> KIPEHLIGKGAEADIKRDSYLDFDVIIKERVKKGYRDERLDENIRKSRTAREARYLALVKDFGIPAPYIFDVDLDNKRIMMSYINGKLAKDVIEDNL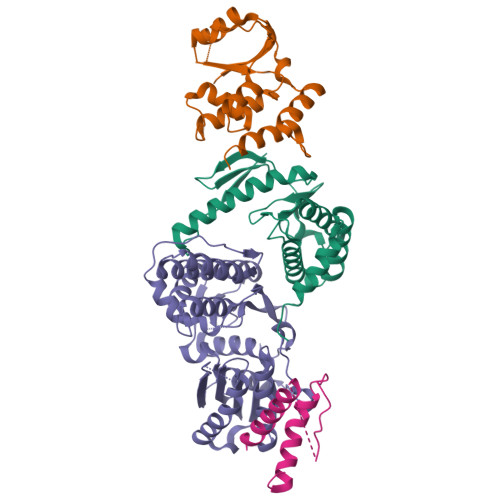DIAYKIGEIVGKLHKNDVIHNDLTTSNFIFDKDLYIIDFGLGKISNLDRDKAVDLIVFKKAVLSTHHEKFDEIWERFLEGYKSVYDRWEIILELMKDVERRARYVE;> PMIIRGIRGARINNEIFNLGLKFQILNADVVATKKHVLHAINQAKTKKPIAKSFWMEILVRASGQRQIHEAIKIIGAKDGNVCLICEDEETFRKIYELIGGEIDDSVLEINEDKERLIREIFKIRGFGNVVERVLEKIALIELKKE;> MICLGLEGTAEKTGVGIVTSDGEVLFNKTIMYKPPKQGINPREAADHHAETFPKLIKEAFEVVDKNEIDLIAFSQGPGLGPSLRVTATVARTLSLTLKKPIIGVNHCIAHIEIGKLTTEAEDPLTLYVSGGNTQVIAYVSKKYRVFGETLDIAVGNCLDQFARYVNLPHPGGPYIEELARKGKKLVDLPYTVKGMDIAFSGLLTAAMRAYDAGERLEDICYSLQEYAFSMLTEITERALAHTNKGEVMLVGGVAANNRLREMLKAMCEGQNVDFYVPPKEFCGDNGAMIAWLGLLMHKNGRWMSLDETKIIPNYRTDMVEVNWI;> MKAKRVQAKIEIEFPSEDVAKVVYEAVLYEHLSVPYRRSEIDFKLEGKKIILDIKATDSSALRGTVNSYLRWIKAAIDVIEV> NRPMETTITRQDIPIEARMNEIVHSLKSRGTRINFMDLFPYEQKEHLVVTFLAVLE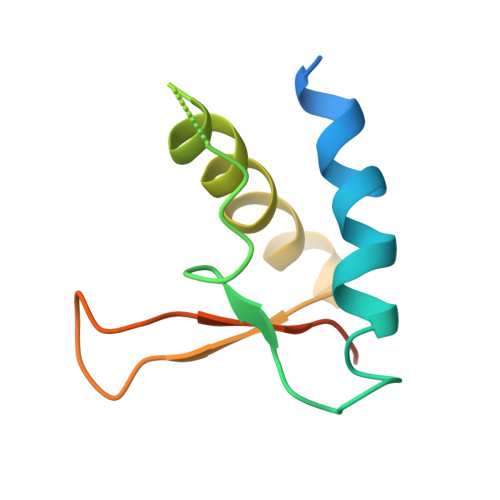LMKNQLVLIEQEHNFSDIYITGSESIHGAVDKL>DSEGGEDEDLQCVCLKTTSGINPRHISSLEVIGAGLHCPSPQLIATLKTGRKICLDQ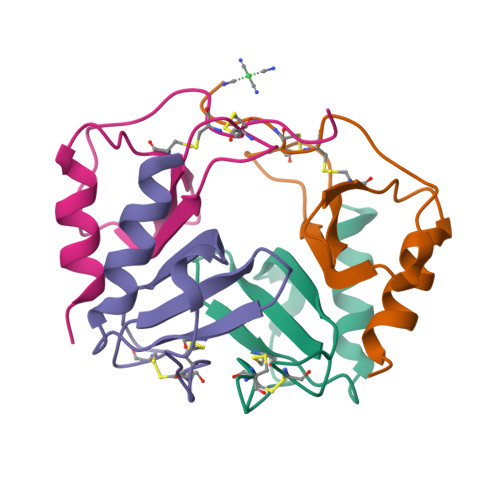QNPLYKKIIKRLLKS[4x]>[4x]MPLSQEESTLIERATATINSIPISEDYSVASAALSSDGR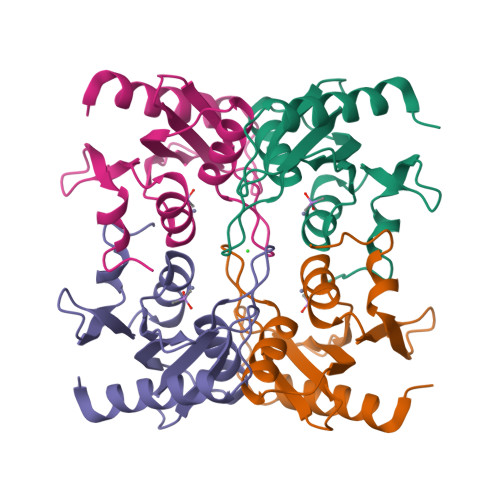IFTGVNVYHFTGGPCAELVVLGTAAAAAAGNLTCIVAIGNENRGILSPCGKCRQVLLDLHPGIKAIVKDSDGQPTAVGIRELLPSGYVWEG> MSALLKEILALTVKSEAALWKGAEQKVLSGLNNLAKTELVQITHHFGVNKQGSEALWSQLDKAAVGAFPELSVDETL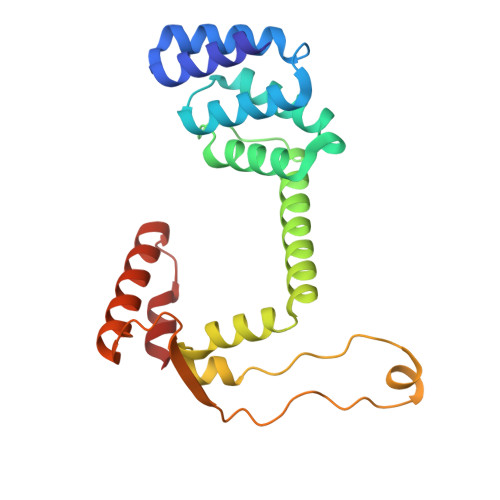QLIDGFGECPDSYTLSHDLNQRLLVSWEQLGKLNFQKLKETNPYFASDIVNQLDAAAAEFIKVRPAAESEAGGFLNSLGVSSSFNTTKNDIYVVQSASGKKLNNKEQREAYVLEKAQKYLKEDPQSKILDIIAQK> P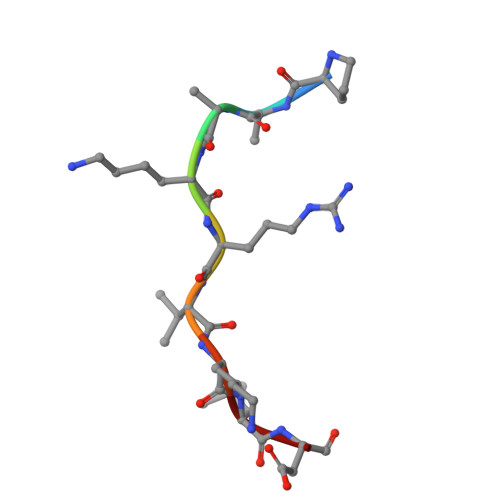AAKRVKLD> ISGGDAIYSSTGRCSLGFNVRSGSTYYFLTAGHCTDGATTWWANSARTTVLGTTSGSSFPNNDYGIVRYTNTTIPKDGTVGGQDITSAANATVGMAVTRRGSTTGTHSGSVTALNATVNYGGGDVVYGMIRTNVCAEPGDSGGPLYSGTRAIGLTSGGSGNCSSGGTTFFQPVTEALSAYGVSVY;> VDCSEYPKPACTPEYRPLCGSDNKTYGNKCNFCNAVVESNGTLTLSHF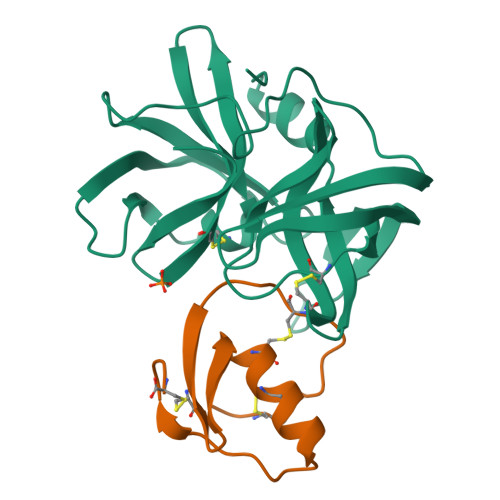GKC BAF is a small (89 amino acid) protein that localizes to the nucleus, at the NE and in the cytoplasm. BAF dimerization allows for its binding to LEM domain proteins and the Ig-fold domain of lamin A/C, while each individual subunit can bind dsDNA. More recently, BAF was found to play a direct role in repairing ruptures of the NE by recruiting LEM domain proteins and membranes to the sites of rupture. Nestor–Guillermo progeria syndrome (NGPS) is caused by a homozygous alanine-to-threonine mutation at position 12 (A12T) in barrier-to-autointegration factor (BAF).

In order to further characterize the effect of the A12T mutation on BAF 3D structure and binding properties, we initiated a structural analysis of BAF A12T by X-ray crystallography. The only interaction known to directly involve alanine 12 is the interaction of BAF with the Ig-fold domain of lamin A/C. Therefore, we determined the 3D structure of BAF A12T bound to the lamin A/C Ig-fold domain at 1.6 Å resolution. Only slight changes in the relative positioning of the BAF monomers, as well as in the structure of some lamin A/C loops (especially at Ser433-Thr434) were observed. We thus concluded that the A12T mutation does not affect BAF 3D structure. Despite an apparent similarity between the 3D structures of the WT and mutated complexes, prediction of the binding energies from these 3D structures using the PDBePISA server suggested that the A12T mutation changes the thermodynamical equilibrium of the system, with the mutant binding with a free energy ΔG that is 1.8 kcal/mol less favourable compared to the WT. Also, both BAF WT and A12T dimers bind to a single Ig-fold domain in the crystal structures. We obtained KD values of 2.7 ± 1.2 μM and 33 ± 4 μM for the interactions involving BAF WT and BAF A12T, respectively, showing that the A12T mutation decreases the affinity of BAF for lamin A/C Ig-fold by about tenfold. In addition, we noticed enrichment of PLA foci in nuclear blebs of a subset of control cells, indicating that blebs could be a site of increased interaction between BAF and lamin A/C. Together these data show that the BAF A12T mutation reduces the affinity of BAF for lamin A/C both in vitro and in NGPS cells. Here, we demonstrated that, in the presence of BAF A12T, lack of A-type lamins accumulation at sites of ruptures does not affect the dynamics of NE repair but leaves areas of the NE devoid of lamin A/C that are more prone to re-rupture.

>GTTSQKHRDFVTEPMGEKPVGSLAGIGEVLGKKLEERGFDKAYVVLGQFLVLKKDEDLFREWLKDTAGANAKQSRDAFGALREWADAFL[4x];>[2x]GGGSVTKKRKLESTESRSSFSQHARTSGRVAVEEVDEEGKFVRLRNKSNEDQSMGNWQIKRQNGDDPLLTYRFPPKFTLKAGQVVTIWAAGAGATHSPPTDLVWKAQNTWGCGNSLRTALINSTGEEVAMRKLVRSVTVVEDDEDEDGDDLLHHHH>SCYFIPNEGVPGDSTRKCMDLKGNKHPINSEWQTDNCETCTCYETEISCCTLVSTPVGYDKDNCQRIFKKEDCKYIVVEKKDPKKTCSVSE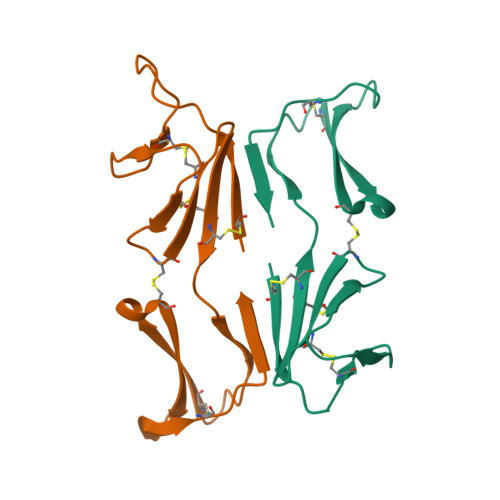WII[4x]>MSKTITYYNSGAVPLINASELPYDVVNLAFLSSSSNNPFNLVLSGAIAATESSFTTNTIEAIKVMQHKGQKV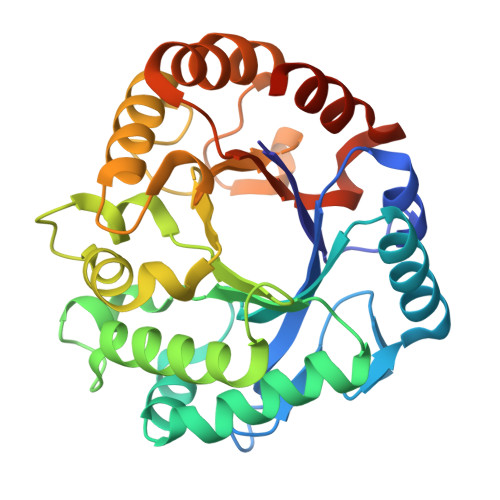LISFGGGTMGSNAYRSLSEDTAKLADSLASFVKNNQLDGVDIDYEDTAAFTGQAGYDGAQFLISLTQELRKRLPSPDYIISHAPQPPYLEQGGYMAGYVEVVELVGQEIDWLNVQFYNNPPWSANPDQIVSSYLNYTKLPNMSPEKVIAGFPVTQNDAGSGYMPVQTIINEVIKPIQQQSSLGGIMNWQFSSDHNGDWIKAIAQSLNSLEHHHHHH[4x]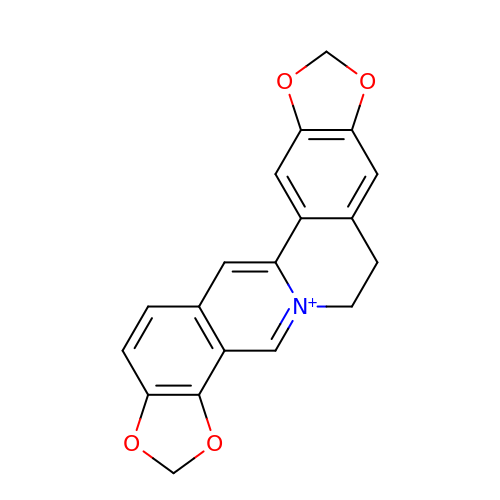6,7-dihydro[1,3]dioxolo[4,5-g][1,3]dioxolo[7,8]isoquino[3,2-a]isoquinolin-5-ium | C19 H14 N O4 | XYHOBCMEDLZUMP-UHFFFAOYSA-N>[2x]GAMAGVFTYETEFTSVIPPPRLFKAFILDADNLIPKIAPQAVKCAEIIEGDGGVGTIKKITFGEGSWFGSVTHKIDGIDKENFVYSYSLIEGDALSDKIEKISYETKLVSSSD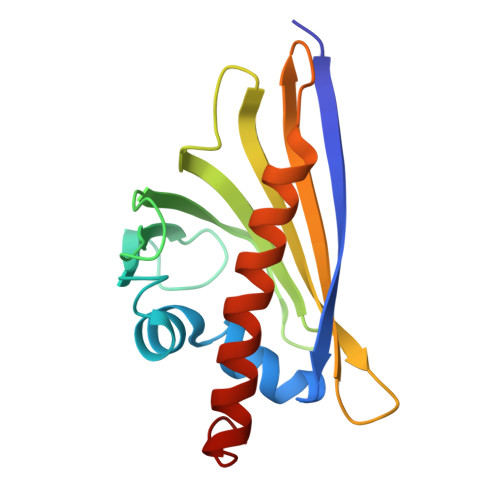GGSIIKSTSNYHTKGDVEIKEEHVKAGKEKASHLFKLVEGYLLANPNEYC> GSMSYD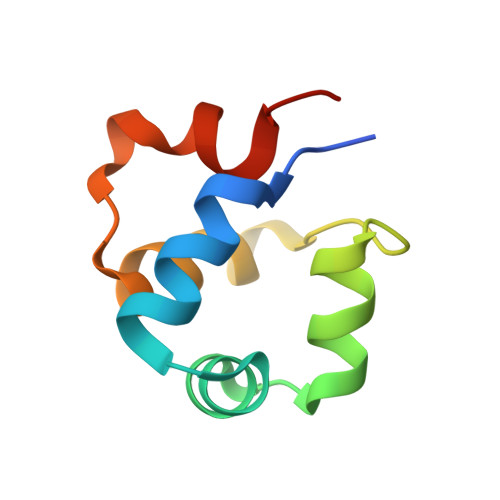YSSLLGKITEKCGTQYNFAIAMGLSERTVSLKLNDKVTWKDDEILKAVHVLELNPQDIPKYFFNAKVH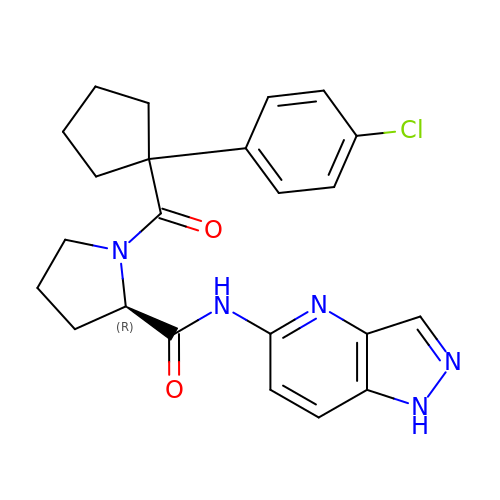1-[1-(4-chlorophenyl)cyclopentane-1-carbonyl]-N-1H-pyrazolo[4,3-b]pyridin-5-yl-D-prolinamide | C23 H24 Cl N5 O2 | IDPXNSVWJPGGFG-LJQANCHMSA-N2-[[3-[[(4~{R})-3,3-bis(fluoranyl)piperidin-4-yl]carbamoyl]phenyl]amino]-~{N}-(2-chloranyl-6-methyl-phenyl)-1,3-thiazole-5-carboxamide 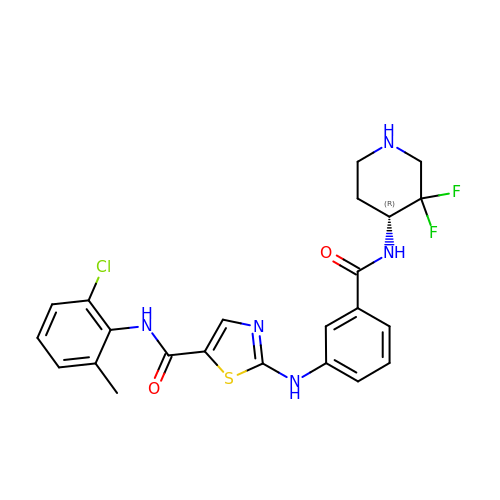| C23 H22 Cl F2 N5 O2 S | HZPGXKUXZFAZJJ-GOSISDBHSA-N>[2x]SRPQSTLRRAITAAYRRPETECLPPLVEAATQSKEIRDAAASTARKLIEALRGKHSGSGSSGSMMGEQFVTGETIREALKRSKELEEKGFSYSYDMLGEAATTAADAERYYRDYESAIHAIGKASAGRGIYEGPGISIKLSALHPRYSRAQAARVMGELLPRVKALALLAKNYDIGLNIDAEEADRL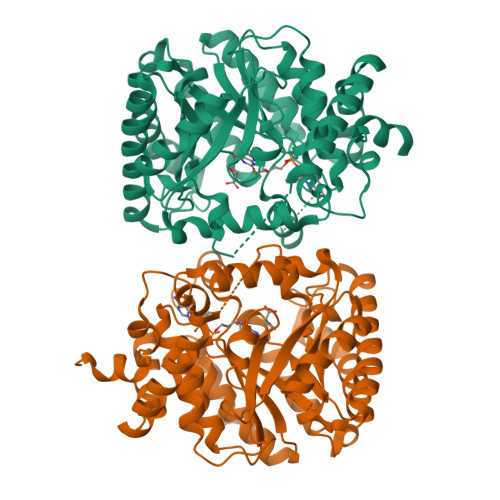ELSLDLLEVLCLDGDLSGWNGMGFVVQAYGKRCPFVLDFIIDLARRSGRRIMVRLVKGAYWDAEIKRAQLDGLADFPVFTRKIHTDVSYIACAAKLLAATDVVFPQFATHNAQTLAAIYHMAGKDFHVGKYEFQCLHGMGEPLYEEVVGRGKLDRPCRIYAPVGTHETLLAYLVRRLLENGANSSFVHRINDPKVSIDELIADPVEVVRAMPVVGAKHDRIALPA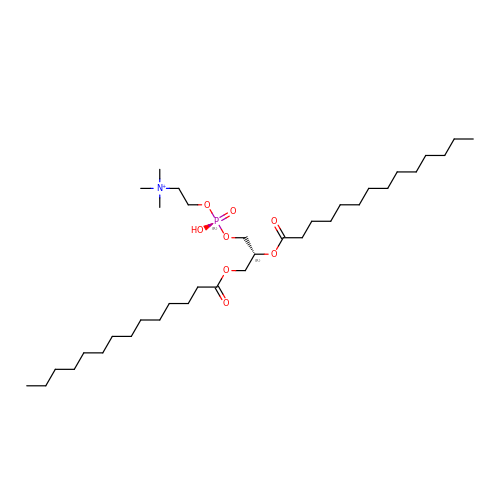1,2-DIMYRISTOYL-SN-GLYCERO-3-PHOSPHOCHOLINE | C36 H73 N O8 P | CITHEXJVPOWHKC-UUWRZZSWSA-O> MAVPETRPNHTIYINNLNEKIKKDELKKSLHAIFSRFGQILDILVSRS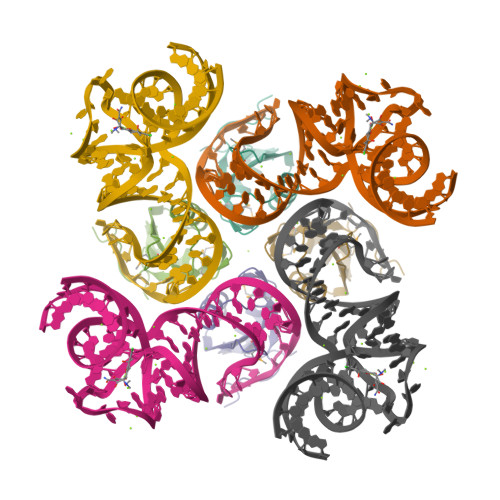LKMRGQAFVIFKEVSSATNALRSMQGFPFYDKPMRIQYAKTDSDIIAKMK>GAMAMSDLPIEFTELVDLMSLGISPQFLDFRSTTFESDHFVTVRETKDGTNSVAIVDLAKGNEVTRKNMGGDSAIMHPSQMVISVRANGTIVQIFNLETKSKLKSFTLDEPVIFWRWLSETTLGFVTARSILTSNVFDGNVNAKPQLLTLRHANLNNTQIINFVANKNLDWFAVVGILQENGRIAGRIQLFSKQRNISQAIDGHVAIFTNILLEGNGSTPVQVFVTGNRNATTGAGELRIIEIDHDASLPSQYQKETTDIFFPPDATNDFPIAVQVSEKYGIIYLLTKYGFIHLYELETGTNLFVNRITAESVFTAAPYNHENGIACINKKGQVLAVEISTSQIVPYILNKLSNVALALIVATRGGLPGADDL[4x];>NLNLIDM[10x]

The protein that gives the process its name, Clathrin, is a triskelion composed of three heavy chains (Clathrin Heavy Chain, Chc) that provide the structural backbone of the lattice, further stabilized and regulated by three light chains (Clathrin Light Chain, Clc). The proximal domain specifically interacts with Clcs, whereas, the N-terminal domain (NTD) of Chc, which adopts a WD40 beta-propeller structure, is pivotal for interactions with various adaptor proteins (APs). To investigate the existence of binding sites present in Clathrin NTD, we crystallized the N-terminal domain of Chc with different peptides derived from adaptor proteins containing CBMs. All our structures show that each peptide binds to three different binding pockets (Clathrin, Arrestin and W-box).

Crystal structure of Chc-NTD (displayed as a grey cartoon) bound to CBMs from Ent1 (1.75 Å, red), Ent2 (1.74 Å, yellow), Ent5 (Ent5.1 LIDL motif, 2.01 Å, green), Apl2.1 (Apl2.1 LLDLF motif, 2.75 Å, blue) and Yap1801 (1.95 Å, grey). Additionally, K98 interacts with position −2 of the motif as observed in the Ent5.1, Apl2.1 and Yap1801 complexes. Residue K284 within the W-box establishes salt bridges with the carboxy-terminal of Ent1, Ent2 and Yap1801. Concurrently, K326 forms hydrogen bonds with the peptide backbone at positions +2, +4 and +1 for the Ent5.1, Apl2.1 and Yap1801 complexes. Water-mediated interactions are also observed in the W-box between the NTD backbone (L24, D25 and V309) and the peptide at position +3, for both Ent1 and Ent2. However, Apl2.1 and Yap1801 do not show density compatible with water molecules near the binding sites. Interestingly, the substitution of the second Leu (LIDL) and/or the addition of non-negatively charged residues at the C-terminal of the CBM decreases the binding affinity. Specifically, the Leu/Ile substitution on Yap1802 retrieves a KDApp≅ 311 µM and the Leu/Met substitution on Yap1801 a KDApp≅ 598 µM.> ALQLWQFLVALLDDPTNAHFIAWTGRGMEFKLIEPEEVARLWGIQKNRPAMNYDKLSRSLRYYYEKGIMQKVAGERYVYKFVCEPEALFSLA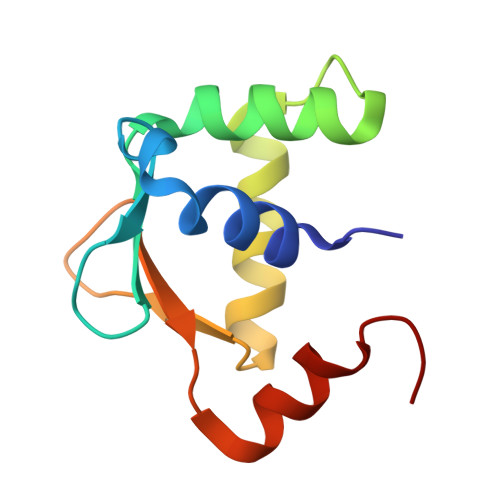FPDNQ N1-(5'-PHOSPHO-ALPHA-RIBOSYL)-5-METHOXYBENZIMIDAZOLE 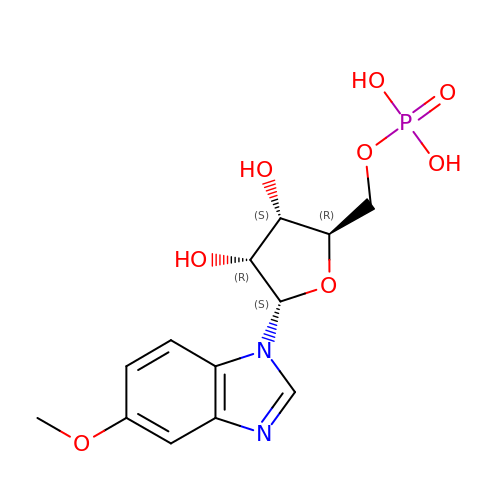| C13 H17 N2 O8 P | VYUPJUKSTVHSQI-LPWJVIDDSA-N> TEEFDAIKIALASPDMIRSWSFGEVKKPETINYRTFKPERDGLFCARIFGPVKDYECLCGKYKRLKHRGVICEKCGVEVTQTKVRRERMGHIELASPTAHIWFLKSLPSRIGLLLDMPLRDIERVLYFESYVVIEGGMTNLERQQILTEEQYLDALEEFGDEFDAKMGAEAIQALLKSMDLEQECEQLREELNETNSETKRKKLTKRIKLLEAFVQSGNKPEWMILTVLPVLPPDLRPLVPLDGGRFATSDLNDLYRRVINRNNRLKRLLDLAAPDIIVRNEKRMLQEAVDALLDNGRRGRAITGSNKRPLKSLADMIKGKQGRFRQNLLGKRVDYSGRSVITVGPYLRLHQCGLPKKMALELFKPFIYGKLELRGLATTIKAAKKMVEREEAVVWDILDEVIREHPVLLNRAPTLHRLGIQAFEPVLIEGKAIQLHPLVCAAYNADFDGDQMAVHVPLTLEAQLEARALMMSTNNILSPANGEPIIVPSQDVVLGLYYMTRDCVNAKGEGMVLTGPKEAERLYRSGLASLHARVKVRITEYEKDANGELVAKTSLKDTTVGRAILWMIVPKGLPYSIVNQALGKKAISKMLNTCYRILGLKPTVIFADQIMYTGFAYAARSGASVGIDDMVIPEKKHEIISEAEAEVAEIQEQFQSGLVTAGERYNKVIDIWAAANDRVSKAMMDNLQTETVINRDGQEEKQVSFNSIYMMADSGARGSAAQIRQLAGMRGLMAKPDGSIIETPITANFREGLNVLQYFISTHGARKGLADTALKTANSGYLTRRLVDVAQDLVVTEDDCGTHEGIMMTPVIEGGDVKEPLRDRVLGRVTAEDVLKPGTADILVPRNTLLHEQWCDLLEENSVDAVKVRSVVSCDTDFGVCAHCYGRDLARGHIINKGEAIGVIAAQSIGEPGTQLTMRTFHIGGAASRAAAESSIQVKNKGSIKLSNVKSVVNSSGKLVITSRNTELKLIDEFGRTKESYKVPYGAVLAKGDGEQVA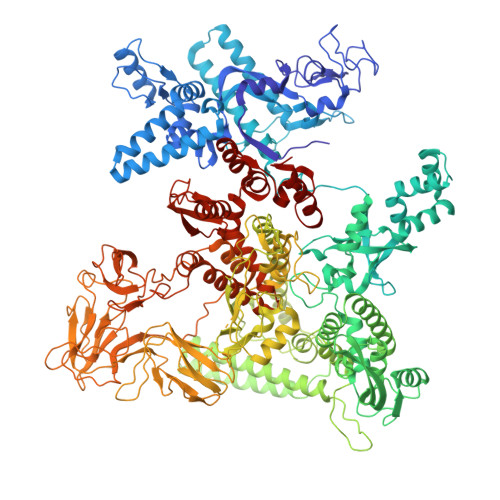GGETVANWDPHTMPVITEVSGFVRFTDMIDGQTITRQTDELTGLSSLVVLDSAERTAGGKDLRPALKIVDAQGNDVLIPGTDMPAQYFLPGKAIVQLEDGVQISSGDTLARIPQESGGTKDITGGLPRVADLFEARRPKEPAILAEISGIVSFGKETKGKRRLVITPVDGSDPYEEMIPKWRQLNVFEGERVERGDVISDGPEAPHDILRLRGVHAVTRYIVNEVQDVYRLQGVKINDKHIEVIVRQMLRKATIVNAGSSDFLEGEQVEYSRVKIANRELEANGKVGATYSRDLLGITKASLATESFISAASFQETTRVLTEAAVAGKRDELRGLKENVIVGRLIPAGTGYAYHQDRMRRRAAG>MQRIIVNPNEPYLSVIKKVVKLSIPIIVVNLLYTVENMISMILVSSISPSAVAATGFSLSLLWFIYSLMALSYSGTNILIAQFVGAKKDPSPILINGLFLSFLISLPLFFYGKDFVLFLMKVLGASETVRSLAKEYLTPIFWFIPIGFLTNTFYGAYNGAGDTKTPMKVAIIMNLTHIGTAYTLINGKFGLPKLGVEGAGWGIAISEILAFFIYTFLLIFFKKPFPLHLRLEPKLLFKMVRLGTPTALERAITTLSFNVFVGFLAKFGDKVLAAHQIGLRIESISFMIGFGVMIASTTLAGQN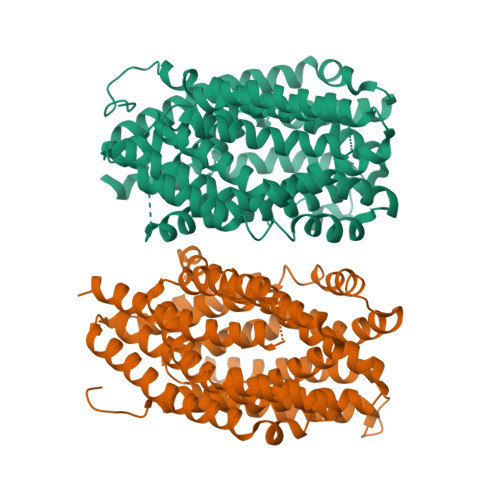YGARNYRGMVHAVNTSAHFTALVMSLTGLILILFPHYLVYPFSRDPEVIEWASYYLQIVGISQPAMAYASIYSGALKGMGKTHIPLFVNISSFWLFRIIPSYFLLKVIHSPLVPWGFMTFETAVRALFYYTVFKKVVGKLLQTFQKEEEPEGEDAEGDKPLDEVRSKVT[2x]>[5x]EAEAADRADILYNIR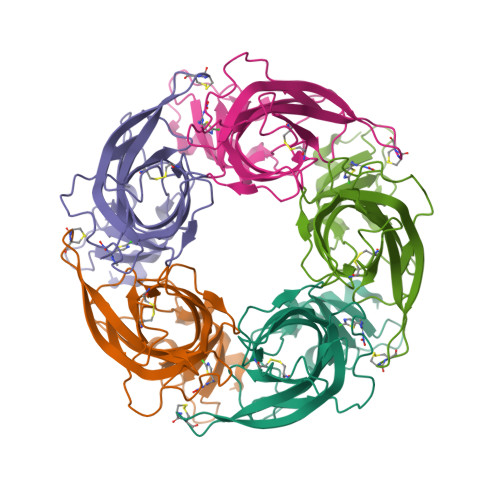QTSRPDVIPTQRDRPVAVSVSLKFINILEVNEITNEVDVVFWQRTTWSDRTLAWDSSHSPDQVSVPISSLWVPDLAAYNAISKPEVLTPQLARVVSDGEVLYMPSIRQRFSCDVSGVDTESGATCRIKIGSWTHHSREISVDPTTENSDDSEYFSQYSRFEILDVTQKKNSVTYSCCPEAYEDVEVSLNFRKKGRSEIL>[2x]TNKEL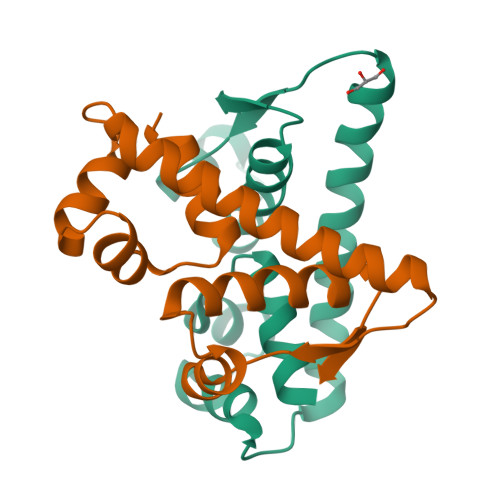QAIRKLLMLDVSEAAEHIGRVSARSWQYWESGRSAVPDDVEQEMLDLASVRIEMMSAIDKRLADGERPKLRFYNKLDEYLADNPDHNVIGWRLSQSVAALYYTEGHADLI>[2x]MKVTI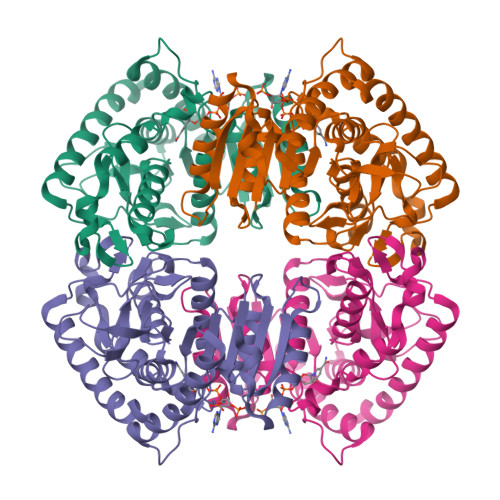IGASGRVGSATALLLAKEPFMKDLVLIGREHSINKLEGLREDIYDALAGTRSDANIYVESDENLRIIDESDVVIITSGVPRKEGMSRMDLAKTNAKIVGKYAKKIAEICDTKIFVITNPVDVMTYKALVDSKFERNQVFGLGTHLDSLRFKVAIAKFFGVHIDEVRTRIIGEHGDSMVPLLSATSIGGIPIQKFERFKELPIDEIIEDVKTKGEQIIRLKGGSEFGPAAAILNVVRCIVNNEKRLLTLSAYVDGEFDGIRDVCIGVPVKIGRDGIEEVVSIELDKDEIIAFRKSAEIIKKYCEEVKNL> APVRSLNCTLRDSQQKSLVMSGPYELKALHLQGQDMEQQVVFSMSFVQGEESNDKIPVALGLKEKNL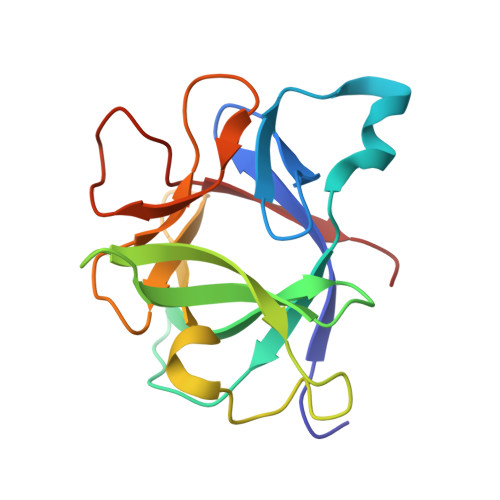YLSCVLKDDKPTLQLESVDPKNYPKKKMEKRFVWNKIEINNKLEFESAQFPNWYISTSQAENMPVFLGGTKGGQDITDFTMQFVSS> MGHHHHHHGGMSNWTTYPQKNLTQAEQLAQLIKEADALVVGIGAGMSAADGFTYIGPRFETAFPDFIAKYQFLDMLQASLFDFEDWQEYWAFQSRFVALNYLDQPVGQSYLDLKEILETKDYHIITTNADNAFWVAGYDPHNIFHIQGEYGLWQCSQHCHQQTYKDDTVIRQMIAEQKNMKVPGQLIPHCPECEAPFEINKRNEEKGMVEDADFHAQKARYEAFLSEHKEGKVLY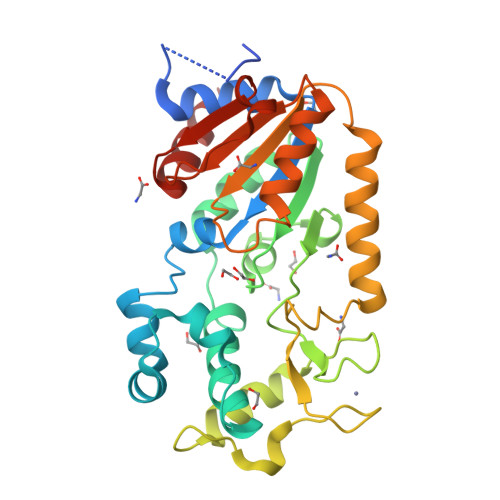LEIGVGHTTPQFIKHPFWKRVSENPNALFVTLNHKHYRIPLSIRRQSLELTEHIAQLISATKTIYQKS> VIGGNECDINEHRFLVAFFNTTGFFCGGTLINPEWVVTAAHCDSTNFQMQLGVHSKKVLNEDEQTRNPKEKFICPNKNNNEVLDKDIMLIKLD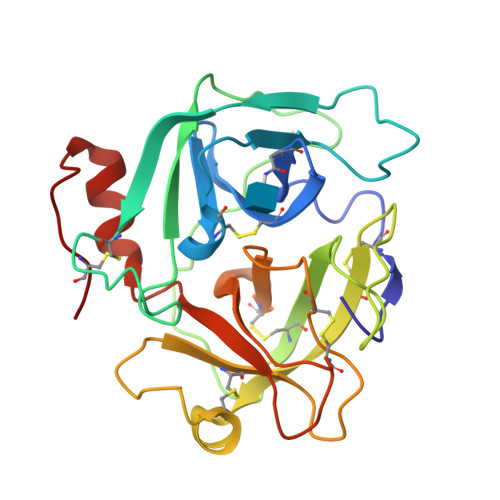KPISNSKHIAPLSLPSSPPSVGSVCRIMGWGSITPVKETFPDVPYCANINLLDHAVCQAGYPELLAEYRTLCAGIVQGGKDTCGGDSGGPLICNGQFQGIVSYGAHPCGQGPKPGIYTNVFDYTDWIQRNIAGNTDATCPP>MESCYNPGLDGIIEYDDFKLNSSIVEPKEPAPETADGPYLVIVEQPKQRGFRFRYGCEGPSHGGLPGASSEKGRKTYPTVKICNYEGPAKIEVDLVTHSDPPRAHAHSLVGKQCSELGICAVSVGPKDMTAQFNNLGVLHVTKKNMMGTMIQKLQRQRLRSRPQGLTEAEQRELEQEAKELKKVMDLSIVRLRFSAFLRASDGSFSLPLKPVISQPIHDSKSPGASNLKISRMDKTAGSVRGGDEVYLLCDKVQKDDIEVRFYEDDENGWQAFGDFSPTDVHKQYAIVFRTPPYHKMKIERPVTVFLQLKRKRGGDVSDSKQFTYYPLVEDKEEVQRKRRKALPTFSQPFGGGSHMGGGSGGAAGGYGGAGGGGSLGFFPSSLAYSPYQSGAGPMGCY[2x]

Mammalian NF-κB is assembled combinatorially from five subunits, p50/NF-κB1, p52/NF-κB2, RelA/p65, c-Rel, and RelB, into homo- and heterodimers which bind to specific DNA sequences, known as κB site or κB DNA. The DD alone mediates protein homo- and heterodimerization; the NTD and DD together are responsible for DNA binding; and the NLS region is flexible in solution and together with the DD forms the binding sites for the inhibitor of NF-κB (IκB) proteins. The mammalian NF-κB p52:p52 homodimer together with its cofactor Bcl3 activates transcription of κB sites with a central G/C base pair (bp), while it is inactive toward κB sites with a central A/T bp. The p50 and p52 subunits bind to a 5 bp half-site (5′-GGGNN-3′), while the RelA and c-Rel subunits prefer a 4 bp half-site (5′-NNCC-3′).

We mutated the central and flanking bps to generate PSel (mutant A/T-centric) (5′-GGGGTAACCCC-3′) and (−1/+1 swap) (5′-GGGGAGTCCCC-3′) DNAs. PSel (mutant A/T-centric) showed twofold reduced reporter activity, while both PSel (−1/+1 swap) and MHC-κB showed drastically reduced transcriptional activity as compared to the natural PSel-κB. However, compared to previously known structures of NF-κB-DNA complexes, two striking differences are observed. One is that all three PSel-κB DNAs exhibited a distinct widening of the minor groove at the two base-steps around the central position 0 (−1 to 0 and 0 to +1), with width of ~7.5 Å (Figure 1E–G1). In the 18 bp long PSel-κB DNA complexes, the NH1 and NH2 groups of Arg52 form H-bonds with both O6 and N7 groups of G at ±3. Throughout our simulations PSel (natural G/C-centric) largely maintained its widened minor groove at the central 0 position, while the minor groove in PSel (mutant A/T-centric) narrowed slightly; PSel (−1/+1 swap) displayed a significantly narrowed minor groove, which became similar to that of MHC-κB DNA recorded in the simulations. (F) Snapshots of PSel (mutant A/T) showing that the cross-strand H-bonds formed by the propeller twist of at +1 position further narrowed the minor groove (indicated by the dashed line in panel (C)). Both RMSD and minor groove width show less structural stability at the central part of PSel (mutant A/T-centric), which may be attributed to the occasionally formed cross-strand H-bonds. On the other hand, the binding to the MHC and mutant A/T-centric PSel DNAs showed a much larger decrease in enthalpy. Notably, we found that the NTD of p52:p52 subunits could make contacts across the central minor grooves when bound to mutant A/T-centric and −1/+1 swap DNAs. Specifically, the clamping conformation enables Lys144 to form cross-strand binding that engages the phosphates at −3/+3 positions in the opposite DNA strands in the mutant A/T and −1/+1 swap DNAs.>MLTMQEIKAHYRFTDEDAELLGSLFPLAETNKERLADQFYDYLLGIPETAEFLKEDLVLQKLKQTHQDWFVSLFAGSYDNRYIHNLQKIGHAHVRVGLNAHYVNVAMNVVRQFTLSIIQDNFPDPEERRQRREAVEKILDINLDIMSASYREEEM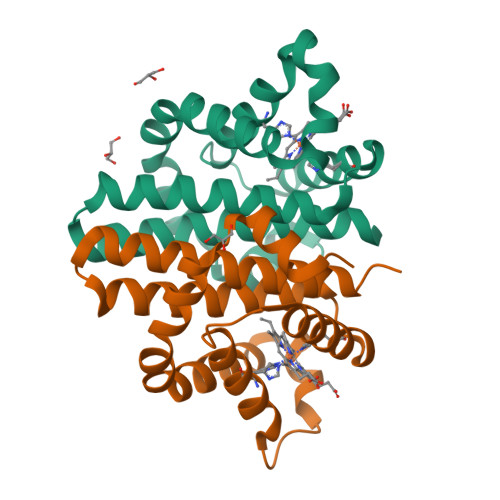RKFFVSH[2x]> GMRRGLVIVGHGSQLNHYREVMELHRKRIEESGAF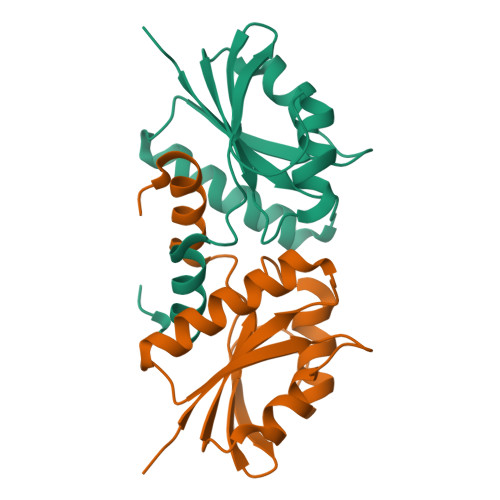DEVKIAFAARKRRPMPDEAIREMNCDIIYVVPLFISYGLHVTEDLPDLLGFPRGRGIKEGEFEGKKVVICEPIGEDYFVTYAILNSVFRIGRDGKGEE N-({4-[4-(2-amino-4-oxo-4,7-dihydro-3H-pyrrolo[2,3-d]pyrimidin-6-yl)butyl]thiophen-2-yl}carbonyl)-L-glutamic acid | C20 H23 N5 O6 S | 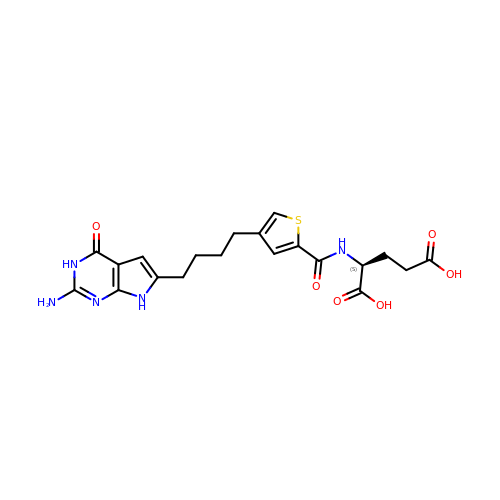VMGGIKVXYOZFJO-ZDUSSCGKSA-N> GPGSRSDSPEIPF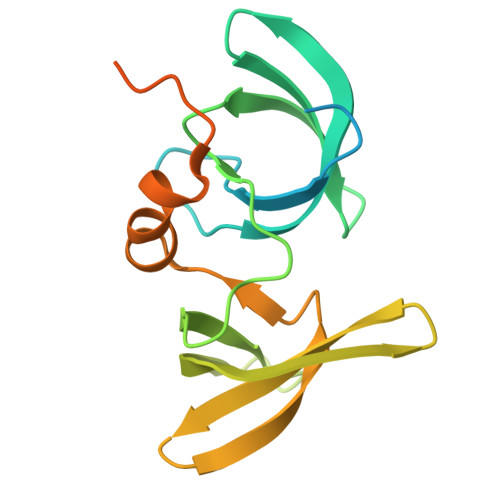QAAAGPSDGLDASSPGNSFVGLRVVAKWSSNGYFYSGKITRDVGAGKYKLLFDDGYECDVLGKDILLCDPIPLDTEVTALSEDEYFSAGVVKGHRKESGELYYSIEKEGQRKWYKRMAVILSLEQGNRLREQYGLGPYEAVTPLTKAADISLDNLVEGKRKRRSNVS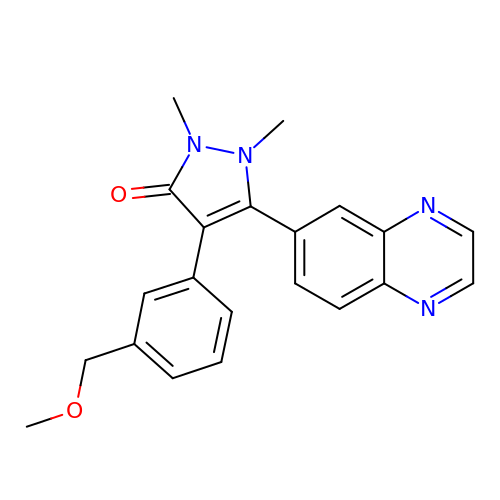4-[3-(methoxymethyl)phenyl]-1,2-dimethyl-5-quinoxalin-6-yl-1,2-dihydro-3H-pyrazol-3-one | C21 H20 N4 O2 | OWJLLMXRMBEWIM-UHFFFAOYSA-N> EKELEPWDLQLQEKESQIQLAESELSLLEETQAKLKKNVETLEEKILAKKTHKQELQDLILDLKKKLNSLKDERSQGEKNFTSAHLKLKEMQKVLNAHRQRAMEARSSLSKAQNKSKVLTALSRLQKSGRINGFHGRLGDLGVIDDSFDVAISTACPRLDDVVVDTVECAQHCIDYLRKNKLGYARFILLDRLRQFNLQPISTPENVPRLFDLVKPKNPKFSNAFYSVLRDTLVAQNLKQANNVAYGKKRFRVVTVDGKLIDISGTMSGGGNHVAKGLMKLGTNQSDKVDDYTPEEVDKIERELSERENNFRVASDTVHEMEEELKKLRDHEPDLESQISKAEMEADSLASELTLAEQQVKEAE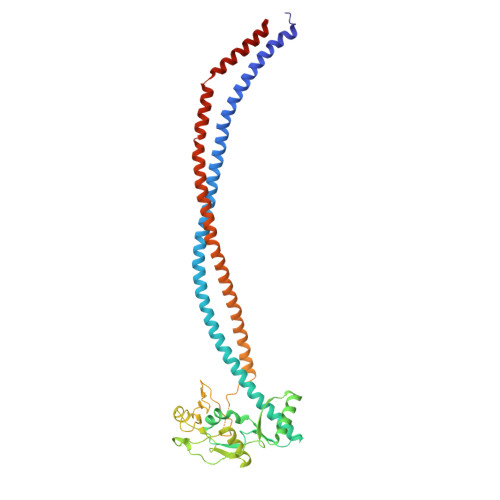MAYVKAVSDKAQLNVVMKNLERLRGEYNDLQSE> MAKLTALTLLGMGLALFDRQKSSFQTRFNVHREVTPVELPNCNLVKGIDNGSEDLEILPNGLAFISSGLKYPGIMSFDPDKSGKILLMDLNEKEPAVSELEIIGNTLDISSFNPQGISTFIDDDNTVYLLVVNQPGSSSTVEVFKFQEE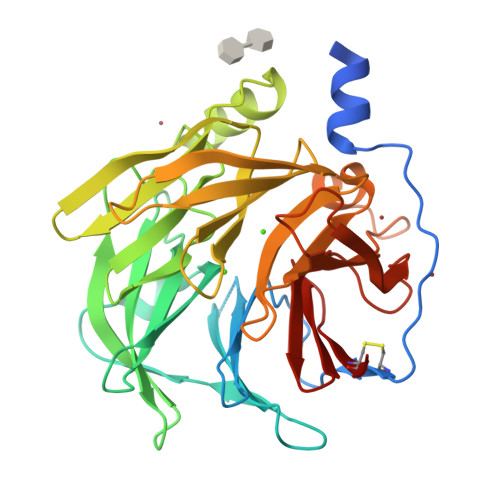EKSLLHLKTIRHKLLPSVNDIVAVGPEHFYATNDHYFIDPYLKSWEMHLGLAWSFVTYYSPNDVRVVAEGFDFANGINISPDGKYVYIAELLAHKIHVYEKHANWTLTPLRVLSFDTLVDNISVDPVTGDLWVGCHPNGMRIFFYDAENPPGSEVLRIQDILSEEPKVTVVYAENGTVLQGSTVAAVYKGKLLIGTVFHKALYCDL> MSILTRWLLIPPVNARLIGRYRDYRRHGASAFSATLGCFWMILAWIFIPLEHP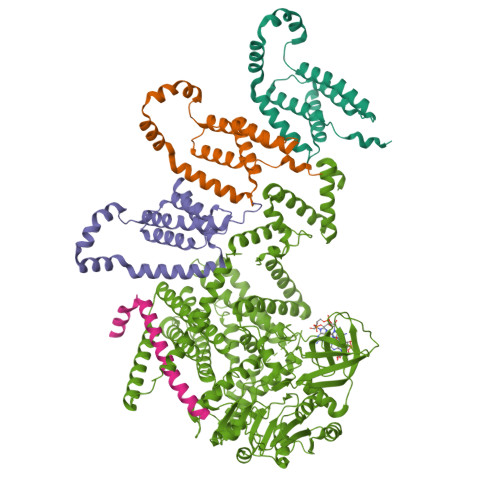RWQRIRAEHKNLYPHINASRPRPLDPVRYLIQTCWLLIGASRKETPKPRRRAFSGLQNIRGRYHQWMNELPERVSHKTQHLDEKKELGHLSAGARRLILGIIVTFSLILALICVTQPFNPLAQFIFLMLLWGVALIVRRMPGRFSALMLIVLSLTVSCRYIWWRYTSTLNWDDPVSLVCGLILLFAETYAWIVLVLGYFQVVWPLNRQPVPLPKDMSLWPSVDIFVPTYNEDLNVVKNTIYASLGIDWPKDKLNIWILDDGGREEFRQFAQNVGVKYIARTTHEHAKAGNINNALKYAKGEFVSIFDCDHVPTRSFLQMTMGWFLKEKQLAMMQTPHHFFSPDPFERNLGRFRKTPNEGTLFYGLVQDGNDMWDATFFCGSCAVIRRKPLDEIGGIAVETVTEDAHTSLRLHRRGYTSAYMRIPQAAGLATESLSAHIGQRIRWARGMVQIFRLDNPLTGKGLKFAQRLCYVNAMFHFLSGIPRLIFLTAPLAFLLLHAYIIYAPALMIALFVLPHMIHASLTNSKIQGKYRHSFWSEIYETVLAWYIAPPTLVALINPHKGKFNVTAKGGLVEEEYVDWVISRPYIFLVLLNLVGVAVGIWRYFYGPPTEMLTVVVSMVWVFYNLIVLGGAVAVSVESKQVRRSHRVEMTMPAAIAREDGHLFSCTVQDFSDGGLGIKINGQAQILEGQKVNLLLKRGQQEYVFPTQVARVMGNEVGLKLMPLTTQQHIDFVQCTFARADTWALWQDSYPEDKPLESLLDILKLGFRGYRHLAEFAPSSVKGIFRVLTSLVSWVVSFIPRRPERSETAQPSDQALAQQGSARSSGRTGLEFEEFYPYDVPDYAADYKDDDDKRS;> TPATQPLINAEPAVAAQTEQNPQVGQVMPGVQGADAPVVAQNGPSRDVKLTFAQIAPPPGSMVLRGINPNGSIEFGMRSDEVVTKAMLNLEYTPSPSLLPVQSQLKVYLNDELMGVLPVTKEQLGKKTLAQMPINPLFITDFNRVRLEFVGHYQDVCENPASTTLWLDVGRSSGLDLTYQTLNVKNDLSHFPVPFFDPRDNRTNTLPMVFAGAPDVGLQQASAIVASWFGSRSGWRGQNFPVLYNQLPDRNAIVFATNDKRPDFLRDHPAVKAPVIEMINHPQNPYVKLLVVFGRDDKDLLQAAKGIAQGNILFRGESVVVNEVKPLLPRKPYDAPNWVRTDRPVTFGELKTYEEQLQSSGLEPAAINVSLNLPPDLYLMRSTGIDMDINYRYTMPPVKDSSRMDISLNNQFLQSFNLSSKQEANRLLLRIPVLQGLLDGKTDVSIPALKLGATNQLRFDFEYMNPMPGGSVDNCITFQPVQNHVVIGDDSTIDFSKYYHFIPMPDLRAFANAGFPFSRMADLSQTITVMPKAPNEAQMETLLNTVGFIGAQTGFPAINLTVTDDGSTIQGKDADIMIIGGIPDKLKDDKQIDLLVQATESWVKTPMRQTPFPGIVPDESDRAAETRSTLTSSGAMAAVIGFQSPYNDQRSVIALLADSPRGYEMLNDAVNDSGKRATMFGSVAVIRESGINSLRVGDVYYVGHLPWFERLWYALANHPILLAVLAAISVILLAWVLWRLLRIISRRRLNPDNE;>[3x]MTQFTQNTAMPSSLWQYWRGLSGWNFYFLVKFGLLWAGYLNFHPLLNLVFAAFLLMPLPRYSLHRLRHWIALPIGFALFWHDTWLPGPESIMSQGSQVAGFSTDYLIDLVTRFINWQMIGAIFVLLVAWLFLSQWIRITVFVVAILLWLNVLTLAGPSFSLWPAGQPTTTVTTTGGNAAATVAATGGAPVVGDMPAQTAPPTTANLNAWLNNFYNAEAKRKSTFPSSLPADAQPFELLVINICSLSWSDIEAAGLMSHPLWSHFDIEFKNFNSATSYSGPAAIRLLRASCGQTSHTNLYQPANNDCYLFDNLSKLGFTQHLMMGHNGQFGGFLKEVRENGGMQSELMDQTNLPVILLGFDGSPVYDDTAVLNRWLDVTEKDKNSRSATFYNTLPLHDGNHYPGVSKTADYKARAQKFFDELDAFFTELEKSGRKVMVVVVPEHGGALKGDRMQVSGLRDIPSPSITDVPVGVKFFGMKAPHQGAPIVIEQPSSFLAISDLVVRVLDGKIFTEDNVDWKKLTSGLHKQHRSPRTQMQ~{N}-[(1~{R},6~{R})-6-azanyl-2,2-bis(fluoranyl)cyclohexyl]-5-ethyl-4-[6-(trifluoromethyl)pyrazolo[1,5-a]pyrimidin-3-yl]thiophene-2-carboxamide 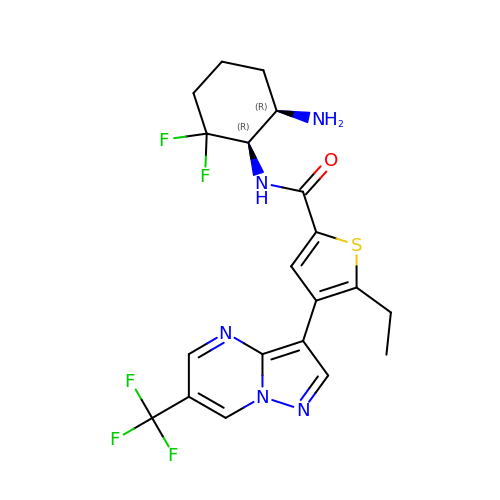| C20 H20 F5 N5 O S | QXXZIVGTJXYLQO-CZUORRHYSA-N N6-{[(3-ethynylphenyl)methoxy]carbonyl}-L-lysine | C16 H20 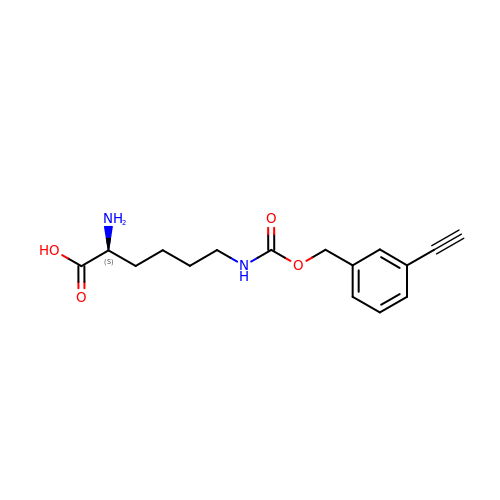N2 O4 | BSKNEGUYHOBMNA-AWEZNQCLSA-N> MSTYYFVIVGQNDNPIYEKEFSTVNKELRKEDHRHLTQFIAHAALDLV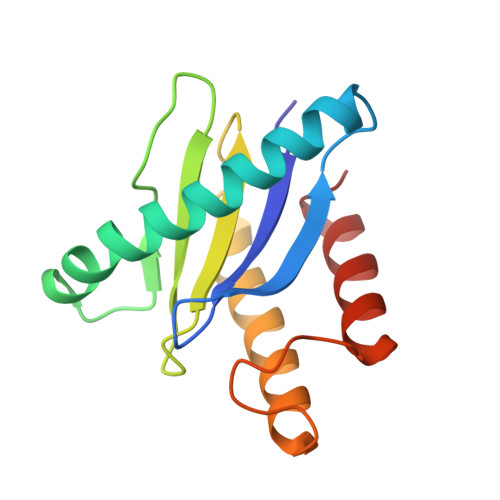DEHKWKTANMQLKSIDRFNQWFVSAFITASQIRFIIVHDNKNDEGIKNFFNEMYDTYIKNSMNAFYRINTPIKSPMFEKKSEIFGRKYLLS>GSAMRSAQVYRWQIPMDAGVVLRDRRLKTRDGLYVCLREGEREGWGEIS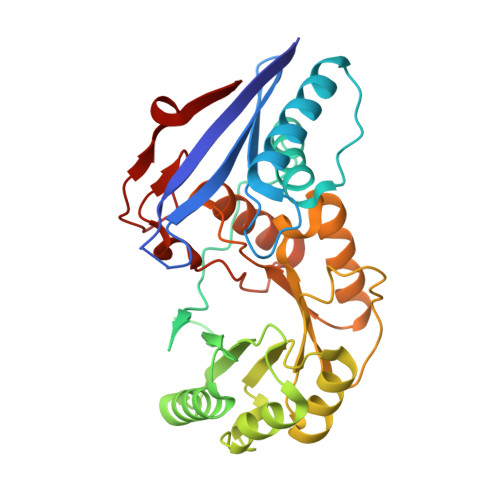PLPGFSQETWEEAQSVLLAWVNNWLAGDCELPQMPSVAFGVSCALAELTDTLPQAANYRAAPLCNGDPDDLILKLADMPGEKVAKVKVGLYEAVRDGMVVNLLLEAIPDLHLRLDANRAWTPLKGQQFAKYVNPDYRDRIAFLAEPCKTRDDSRAFARETGIAIAWDESLREPDFAFVAEEGVRAVVIKPTLTGSLEKVREQVQAAHALGLTAVISSSIESSLGLTQLARIAAWLTPDTIPGLDTLDLMQAQQVRRWPGSTLPVVEVDALERLL[4x]> MGSSHHHHHHENLYFQGGVQIQGHYELKFEAVREAFAALFDDPQERGAGLCIQVGGETVVDLWAGSADKDGREAWHSDTIANLFSCTKTFTAVTALQLVGEGKLSLDAPVVRYWPEFGQAGKASVTLRQLL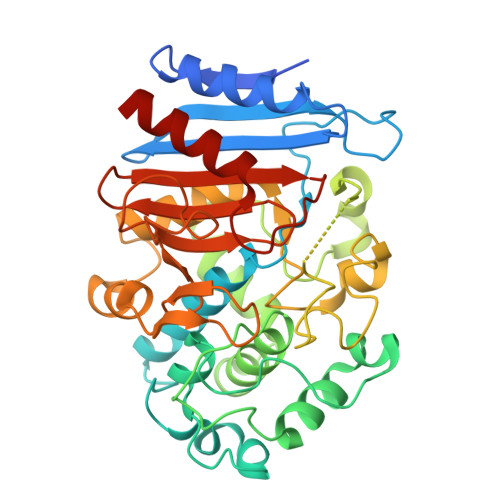SHRAGLPAIRELLPAEALYDWQAMVDALAAEAPWWTPGTEHGYAAITYGWLIGELIRRVDGRGPGESIVARTARPLGLDFHVGLADEEFHRVAHIARGKGNPGDAAAQRLLQVTLREPEALSTRAFTNPPAILTSTNKPEWRRMQQPAANGHGNARSLAGFYAGLLDGSLLESELLDELTREHSLGQDRTLLTQTRFGLGCMLDQPDVANATFGLGARAFGHPGAGGSVGFADPEYDVAFGFVTNTLGPYVLMDPRAQKLVRVLGTCLRRRRR> DDWNWEV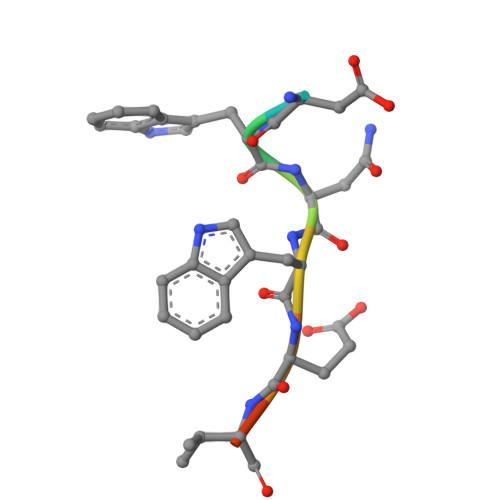ED>MAPSMIPFTIKLKTCLKMCIQRLRYAQEKQQAIAKQSRRQVAQLLLTNKEQKAHYRVETLIHDDIHIELLEILELYCELLLARVQVINDISTEEQLVKEHMDDGINEAIRSLIYAILFVDEVKELSQLKDLMAW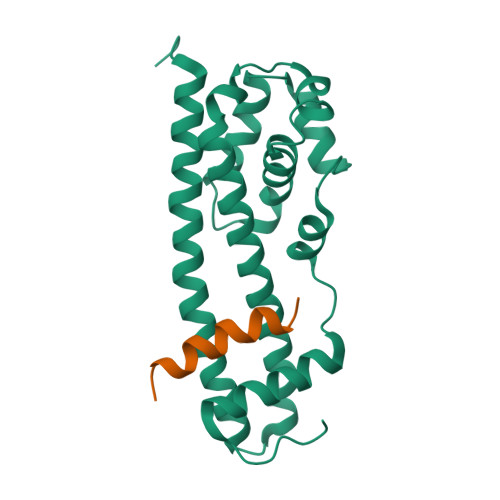KINVEFVNGVIADHIDVPEKIIKKCSPSVPKEELVDLYLKEIAKTYDVPYSKLENSLSS[4x];>NVPEIKAKEVNVDDEKEDKLAQRLRALRG[4x]> MPSEQRGQHRSGYGLGLSTRTQVTGYQFLARRTAMALTRWRVRMEVEPGRRQVLAVVASVSAAGVICLGALLWSFISPSGQMGESPIIADRDSGALYVRVGDTLYPALNLASARLIAGRAENPHKVRSSQIAEQPHGPMVGIPGAPSDISPTSPASSSWLVCDAVTAAQGVGAPASVTVTVIDGTPDLSGRRHVLSGSDAVVLRYGNDTWVIRQGRRSRIDAANRAVLLPLGLTPEQVKQASPMSRALYDALPVGPELAVPKVPDAGKPANFPGAPAPVGAVLVTPQISGPQQYSVVLPDGVQTISPIVAQILQNAGTPAGSMPVVVAPATLARMPVVHGLDLSAYPDSPLNVVNMKENPATCWWWEKTAGEERARTQVVSGPTVP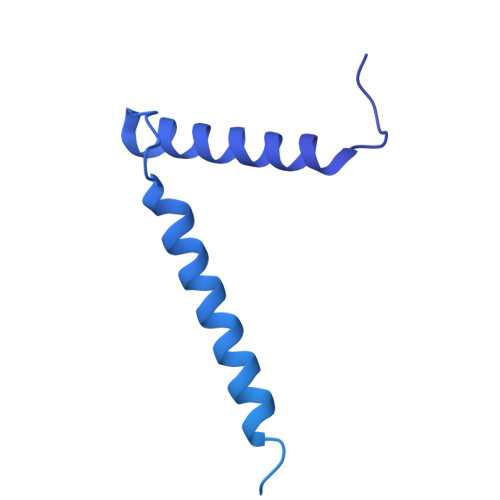IATSDTNKVVSLVKADNTGREADRVYYGPNYANFVVVTGNDPAASTAESLWLLSKSGVRFGVDNSREARTALGLTSTPSPAPWVALRLLAPGPMLSRADALVRHDTLPTDTNPAELAVPK>[2x]MKDIAIRGYCDRPSVATGETIRFYVSANETRGTFDAELVRLIHGDSNPAGPGYKEEAIKSDLEGQYPARFQRTQFGSYVEVADPDAGLQPDGAFSVHLFLWSTTPSRGRQGIASRWNDERQSGWNLAIEDGRVVFTIGDGSGATSSVVSDRPLFQQIWYSITGVYDPEKKQLRLYQKSVVNRTNSRFGLVVPLDSDCAVSADATVKAADSETSLLIAGLGEAAAQDGRTWCIAHYNGKVDAPKIYGCALGQDDAEKLSRGEIVRPISRLAHWDFSAGIGLNGIPTDHVVDASGYGHHGRCMNQPSRGSTGWNWDGHEENFIHCPEQYGALWFHEDCLDDCRWEKDFEFTVPEGLKSDFYAVKIRYEDTEDYIPFFVLPPRGTATAPILVIASTLSYLAYANEQIMHKADIGQAVAGHTPVLNENDVELHKNLSYYGLSTYDGHIDGRGVQYTSWRRPIMNLRPKHRQGFGSIWELPADLHLIDWLNHNGFEYDVATEHDLNDQGAE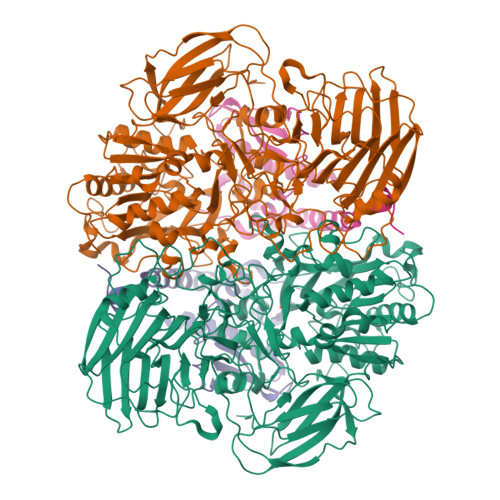LLRRYKVVLTGSHPEYQTWANADAWEDYLADGGRGMYLAANGMYWIVEVHPEKPWVMEVRKELGVTAWEAPPGEYHYSTNGRRGGRFRGRARATQKIWGTGMSSFGFDHSGYFVQMPDSQDERVAWIMEGIDPEERIGDGGLVGGGAGGYELDRYDLALGTPPNTLLLASSVEHSVVYTVIPDDKAFPHPGMNGGEHPFVRADITYFSTANGGGMFATSSISWLGSLSWNDYDNNVSKMTKNVLNQFIKDEPAPRVKLAAALEHHHHHH;>MTEASESCVRDPSNYRDRSADWYAFYDERRRKEIIDIIDEHPEIVEEHAANPFGYRKHPSPYLQRVHNYFRMQPTFGRYYIYSEREWDAYRIATIREFGELPELGDERFKTEEEAMHAVFLRRIEDVRAELA[2x]> UCCCAGUCCACCG;> CGGUGAAAAGGG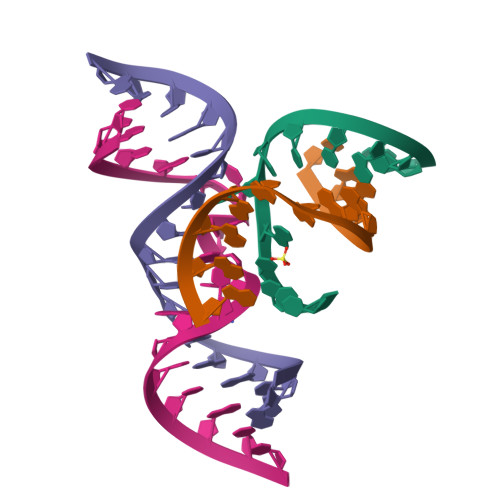;> GGCAGAGAAACACACGA;> UCGUGGUACAUUACCUGCC Mature FP2 is a 27 kDa papain-type protease responsible for cleaving haemoglobin to small peptides, with 93% sequence identity to FP2′ and 68% to parasite falcipain-3. As well as having haemoglobinase activity, FP2 is involved in degrading the erythrocyte skeletal protein ankyrin in a process necessary for red blood cell rupture at the end of the parasite intra-erythrocytic cycle. Similar to other members of the papain protease family, FP2 comprises two distinct sub-domains with primarily α-helical and β-stranded composition, respectively. The substrate cleft and the catalytic site are located between these sub-domains.

Crystals of recombinant mature FP2, lacking the inhibitory pro-domain and with the catalytic site cysteine substituted by alanine for increased stability, were soaked with two previously identified (E)-chalcone molecules, EC54, which exhibited the most potent purely competitive inhibition among derivatives in this earlier study, and EC48. The FP2-EC48 structure, resolved by molecular replacement, revealed two FP2 copies per asymmetric unit of the crystal. Both protein copies exhibited bound EC48 inhibitor (see below) and had nearly identical tertiary structure, with root-mean-square-deviation (RMSD) of Ca atoms below 0.1 Å. EC48 locates in a position distinct from the FP2 catalytic site. Analysis of the structure suggests that EC48 binding is mediated by hydrophobic and π-stacking interactions between the benzodioxol group of the inhibitor (demarcated #1 in the inhibitor structure) and the W449 sidechain of FP2. Further, the inhibitor ketone O (#2 in Fig. 2a) is oriented in a manner that would allow hydrogen bonding to the FP2 C282 backbone O and N, and the Q279 sidechain Nε2, although the distances between these atoms (3.7, 4.3 and 4.4 Å, respectively) suggest any hydrogen bonds would be weak and mostly electrostatic in character. In addition, the structure provides a mechanism for the observed mixed inhibition of FP2 by EC48, as the molecule occupies part of the substrate binding cleft, thereby competing with substrates, and locates just 5.1 and 7.5 Å away from the FP2 H417 and C285, respectively, which comprise the catalytic dyad. In contrast, EC48 occupies the middle of the substrate cleft via its nitrobenzene group and binds to the rear of the cleft via its benzodioxol group. The structure shows that EC48 binds only to the rear of the FP2 substrate cleft, thereby mimicking interactions formed by the L2 loop of naturally occurring, protein-based inhibitors of FP2.

>[2x]GPQMNYEEVIKKYRGEENFDHAAYDWRLHSGVTPVKDQKNCGSAWAFSSIGSVESQYAIRKNKLITLSEQELVDCSFKNYGCNGGLINNAFEDMIELGGICPDGDYPYVSDAPNLCNIDRCTEKYGIKNYLSVPDNKLKEALRFLGPISISVAVSDDFAFYKEGIFDGECGDQLNHAVMLVGFGMKEIVNPLTKKGEKHYYYIIKNSWGQQWGERGFINIETDESGLMRKCGLGTDAFIPLI>[2x]MAKLTIESMPLSVAEGKEVLLLVHN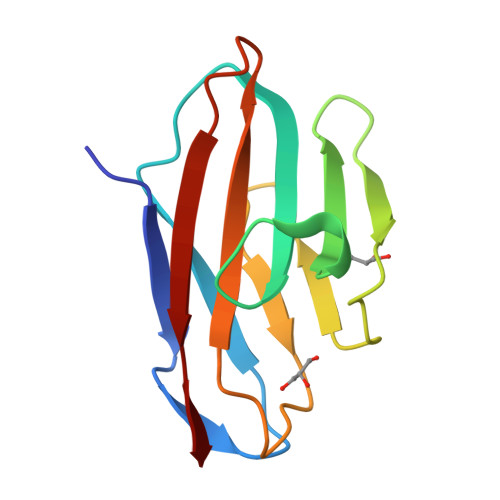LPQHLFGYSWYKGERVDGNSLIVGYVIGTQQATPGAAYSGRETIYTNASLLIQNVTQNDIGFYTLQVIKSDLVNEEATGQFHVY>GKRVLIVDDAAFMRMMLKDIITKAGYEVAGEATNGREAVYKYKELKPDIVTMKITMPEMNGIDAIKEIMKIDPNAKIIVCSAMGQQAMVIEAIKAGAKDFIV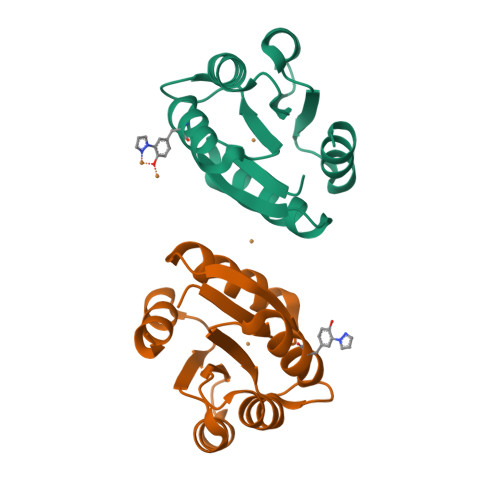KPFQPSRVVEALNKVS[2x]> AVNGTSQFTCFYNSRANISCVWSQDGALQDTSCQVHAWPDRRRWNQTCELLPVSQASWACNLILGAPDSQKLTTVDIVTLRVLCREGVRWRVMAIQDFKPFENLRLMAPISLQVVHVETHRCNISWEISQASHYFERHLEFEARTLSPGHTWEEAPLLTLKQKQEWICLETLTPDTQYEFQ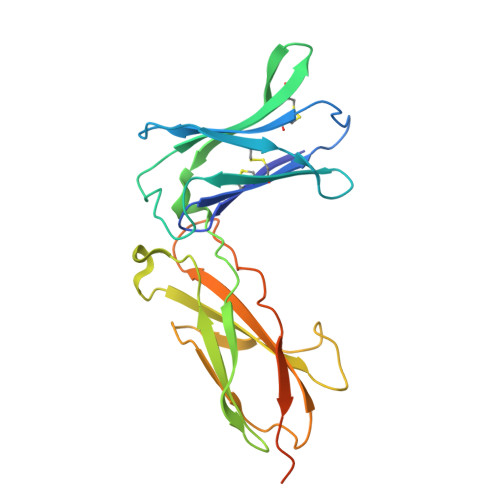VRVKPLQGEFTTWSPWSQPLAFRTKPAALGKDTGAQDKTHTCPPCPAPELLG>LPTQASHNAQPVINLGYARYQGVRLEAGVDEFLGMRYASPPIGDLRFRAPQDPPANQTLQSATEYGPICIGLDEEESPGDISEDCLFINVFKPSTATSQSKLPVWLFIQGGGYAENSNANYNGTQVIQASDDVIVFVTFNYRVGALGFLASEKVRQNGDLNAGLLDQRKALRWVKQYIEQFGGDPDHIVIHGVSAGAGSVAYHLSAYGGKDEGLFI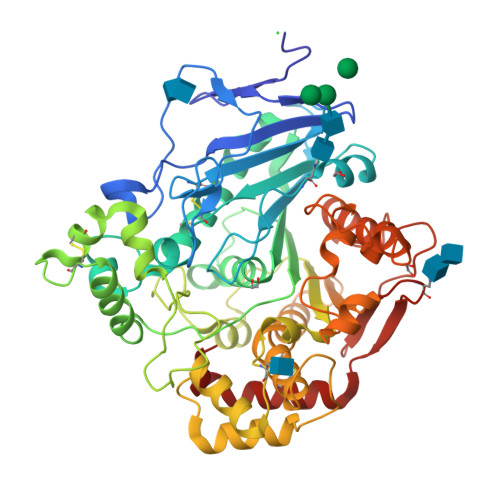GAIVESSFWPTQRTVSEMEFQFERFVNDTGCSSARDSLECLREQDIATIQKGNTGSPFPGGSSSPLPDWYFLPVTDGSLVPDELYNAFDAGNFIKVPVLVGDDTDEGSNFAYNASSSADVSRFFKNNYPNLTSQQLNEINQVYPRGKLLPRHAAYFGASSAAYGDATFTCPGNHVASSAARYLPNSVWNYRVNIIDESNIAGGIGVPHTFELPAIFGAGSTGTLSSDSSYLTYNAAIIPVTMHYFISFVQTLNPNTYRYATAPEWNTWGNGQRLRLQTNDTAMEAVPESSLQDCAFWKSLTVPMEV[2x]> APSPTAPEQPVDVEVQDLEEFALRPAPQGITIKCRITRDKKGMDRGMFPTYFLHLDRED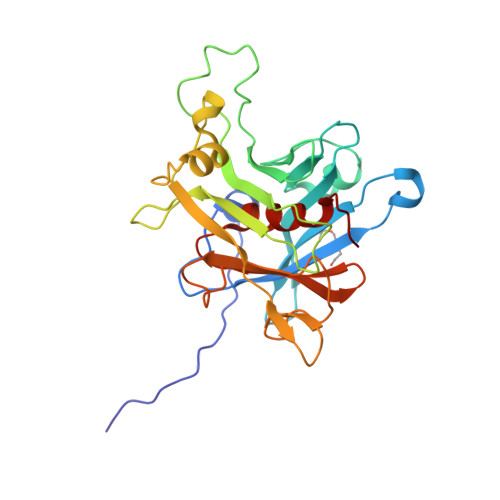GKKVFLLAGRKRKKSKTSNYLISVDPTDLSRGGDSYIGKLRSNLMGTKFTVYDNGVNPQKASSSTLESGTLRQELAAVCYETNVLGFKGPRKMSVIVPGMNMVHERVSIRPRNEHETLLARWQNKNTESIIELQNKTPVWNDDTQSYVLNFHGRVTQASVKNFQIIHGNDPDYIVMQFGRVAEDVFTMDYNYPLCALQAFAIALSSFDSKLACE>GPMANNSVMMKKKLEGKVAIVTGGASGIGEATARLFVKYGARAVVIADIQSELGRSVAESIGKERCSFVQCDVADEEQVKSMIEWTATTYGGLDVMFSNAGVLNSAAQTVKDLDLPLFDKVMRVNTRGAAVCVKQAARKMVELGRGGSIICNAGSSAVRGAHGVTDYVMSK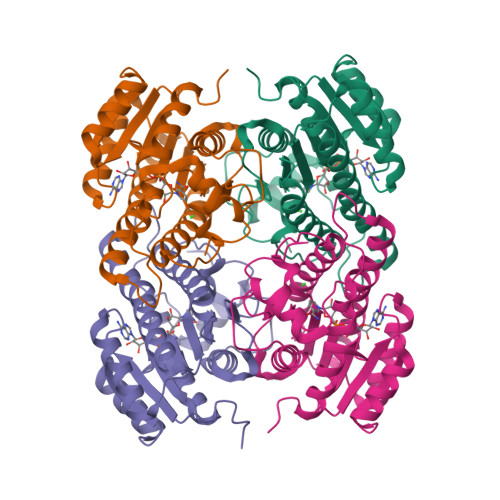HAVIGLVRSASMQLGAHSIRVNSVSPMAVATPLTRNQGISTPDDVQKFLMPFISLKGVPPTAEQVAEAAAFLGSDEAAFVTGHDLPVDGGVLCMPFLLGSA[4x]In order to investigate the influence of metal ions on RNA structure, six octameric RNA duplex structures were solved in the presence of different metal ions. The RNA forms a continuous helix throughout the lattice by end-to-end stacking of the asymmetric unit, as it is often seen in crystal structures of nucleic acids to maximize the energy of the base-stacking. The isomorphous structures showed the characteristics of the A-form helix. In every solved octameric structure one cation is located in the center of the major groove.

The first crystal structure solved by native-SAD was co-crystallized with Ca2+. From the crystal structure in the presence of Ca2+ we could collect a high quality and redundant data set to get sufficient anomalous signal to solve the crystal with native-SAD (single-wavelength anomalous diffraction). In addition to the innersphere binding to the phosphate oxygen of guanine, there is an uncommon innersphere binding to O4 of uracil by Ca2+, Co2+, and Cu2+. Our study also confirms the preference of Tb3+, Ca2+, and Sr2+ to phosphate oxygens, as well as Co2+ and Cu2+ coordination to N7 of guanine, although in an outer-sphere manner in this octameric RNA duplex. Further, an additional Ca2+ is found at the phosphate backbone, reflecting the preference of the bigger-sized Ca2+ for this position. The dominant localization of Ca2+ at phosphate groups corresponds to reported increased stability constants for Ca2+ binding to the phosphodiester bridge. Cu2+, Co2+, and Mn2+ seem to favor binding to the nucleobases, in contrast to Sr2+ or Ca2+. The first is coordinated to the phosphate backbone, the second cation binds in the major groove of the RNA, interacting by a particular innersphere coordination to O4 of uracil in the presence of Ca2+, Co2+, and Cu2+.

>[2x]UCGUACGA LIPOIC ACID | C8 H14 O2 S2 | 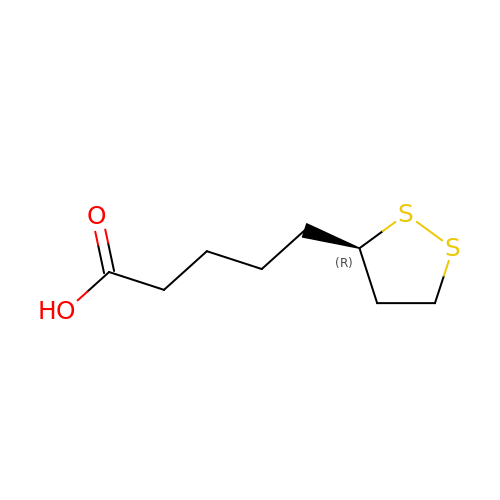AGBQKNBQESQNJD-SSDOTTSWSA-N>[4x]MDYTPHTEEEIREMLRRVGAASLEDLFAHLPKEILSPPIDLPEPLPEWKVLEELRRLAAQNLPAHKAFLGGGVRSHHVPPVVQALAARGEFLTAYTPYQPEVSQGVLQATFEYQTMIAE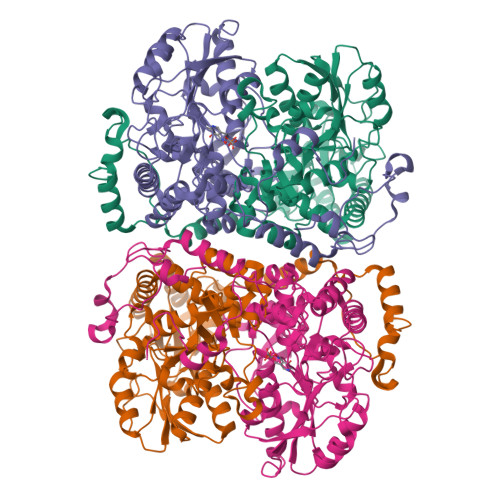LAGLEIANASMYDGATALAEGVLLALRETGRMGVLVSQGVHPEYRAVLRAYLEAVGAKLLTLPLEGGRTPLPEVGEEVGAVVVQNPNFLGALEDLGPFAEAAHGAGALFVAVADPLSLGVLKPPGAYGADIAVGDGQSLGLPMGFGGPHFGFLATKKAFVRQLPGRLVSETVDVEGRRGFILTLQAREQYIRRAKAKSNITTNAQLTALMGAMYLAALGPEGLREVALKSVEMAHKLHALLLEVPGVRPFTPKPFFNEFALALPKDPEAVRRALAERGFHGATPVPREYGENLALFAATELHEEEDLLALREALKEVLA;>[4x]MSFPLIFERSRKGRRGLKLVKAVPKAEDLIPKEHLREVPPRLPEVDELTLVRHYTGLSRRQVGVDTTFYPLGSCTMKYNPKLHEEAARLFADLHPYQDPRTAQGALRLMWELGEYLKALTGMDAITLEPAAGAHGELTGILIIRAYHEDRGEGRTRRVVLVPDSAHGSNPATASMAGYQVREIPSGPEGEVDLEALKRELGPHVAALMLTNPNTLGLFERRILEISRLCKEAGVQLYYDGANLNAIMGWARPGDMGFDVVHLNLHKTFTVPHGGGGPGSGPVGVKAHLAPYLPVPLVERGEEGFYLDFDRPKSIGRVRSFYGNFLALVRAWAYIRTLGLEGLKKAAALAVLNARYLKELLKEKGYRVPYDGPSMHEFVAQPPEGFRALDLAKGLLELGFHPPTVYFPLIVKEALMVEPTETEAKETLEAFAEAMGALLKKPKEWLENAPYSTPVRRLDELRANKHPKLTYFDEG> 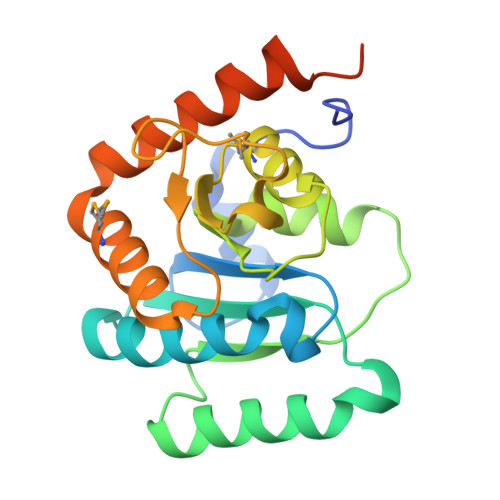SNAHGVDTQVFYPAENRQQQWQDKKIPGKYGIGIFGRIRKTKGTQEFIEAAIVTLKKYPDWTAVVIGEATPRDLDFKKELEQKVKQAGLDKQIIFIGFIADSNEIPSWYRALDIVVCASHKEGFGLPALEAMASKCAVIATKAGAWPEIIVDDENGYLVEPKSSQQIADKLDMLISDSKLRYKIAQNGYDLVTTKYKIQNEAEGIQQVYDRLLAKKRS A large number of double-stranded DNA viruses, including tailed bacteriophages and herpes viruses, use a homomeric ring ATPase to processively translocate viral genomic DNA into procapsids during assembly. By contrast, pac systems feature imprecise, sequence-independent cleavage of the DNA concatemer during head filling, giving rise to variable genome lengths inside virus particles. Both systems encode a large terminase (TerL) protein, composed of a viral packaging ATPase domain and a nuclease domain, and a small terminase (TerS) protein, which recognises the cos or pac site between genome copies and, upon binding of DNA, recruits TerL to make an initiating DNA cut. Here, we reconstituted in vitro a cos packaging system based on bacteriophage HK97 and provided a detailed biochemical and structural description. Crystal structures of the large terminase and DNA-recruiting small terminase, a first for a biochemically defined cos system, reveal mechanistic similarities between cos and pac systems.

By size exclusion chromatography with multi-angle laser-light scattering (SEC-MALS) and native mass spectrometry, the HK97 TerS measured 160.5 kDa and 165.020 ± 0.005 kDa, respectively, in mass, corresponding to an oligomer of nine 18.3-kDa subunits. By X-ray crystallography, we determined the structure of the protein to 1.4 Å resolution. The protein crystallized with three subunits in the asymmetric unit around a crystallographic 3-fold axis, ultimately forming a 9-subunit circular oligomer, in agreement with the biophysical measurements. Of the 161 residues in each protein chain, residues 21–124 had well-resolved electron density. The N-terminal region superposes loosely with the α2 and α3 helices of the helix-turn-helix (HTH) motif of pac phage SF6 GP1 (73), the winged HTH domain of cos phage lambda gpNu1 (74), and the N-terminal HTH motif of cos phage PaP3 TerS. Two strong helix-breaking proline residues, P28 and P29, prevent an α1 helix from forming in the HK97 protein. Following the N-terminal region, two long helices form the basis of oligomerization for the HK97 TerS oligomer. The HK97 oligomer has a van der Waals outer diameter of roughly 85 Å, with an inner tunnel 55 Å long and 18 Å wide at its narrowest point. Residues K36, K37, R47, K77 and K81 form a positive belt around the outside of the complex. However, positive charges from R86, K96, K100, R107 and R114 also line the inner tunnel, which is solvent-exposed and almost wide enough to accommodate double-stranded DNA.

>[3x]ADKRIRSDSSAAAVQAMKNAAVDTIDPPSHAGLEKKAEPFWHDNIRSKALDSWTPADLLAAVELANNQLYITVLRKDLRKEERIRGEERDEGLIKDLRKQIVELQRTILAQRRDLQIHSHATNGESRDQKKRNQNDRDARNTKNEHQDQDDNLIAFPKHG>MSGLADASGPRDTQALLSATQAMDLRRRDYHMERPLLNQEHLEELGRWGSAPRTHQWRTWLQCSRARAYALLLQHLPVLVWLPRYPVRDWLLGDLLSGLSVAIMQLPQGLAYALLAGLPPVFGLYSSFYPVFIYFLFGTSRHISVGTFAVMSVMVGSVTESLAPQALNDSMINETARDAARVQVASTLSVLVGLFQVGLGLIHFGFVVTYLSEPLVRGYTTAAAVQVFVSQLKYVFGLHLSSHSGPLSLIYTVLEVCWKLPQSKVGTVVTAAVAGVVLVVVKLLNDKLQQQLPMPIPGELLTLIGATGISYGMGLKHRFEVDVVGNIPAGLVPPVAPNTQLFSKLVGSAFTIAVVGFAIAISLGKIFALRHGYRVDSNQELVALGLSNLIGGIFQCFPVSCSMSRSLVQESTGGNSQVAGAISSLFILLIIVKLGELFHDLPKAVLAAIIIVNLKGMLRQLSDMRSLWKANRADLLIWLVTFTATILLNLDLGLVVAVIFSLLLVVVRTQMPHYSVLGQVPDTDIYRDVAEYSEAKEVRGVKVFRSSATVYFANAEFYSDALKQRCGVDVDFLISQKKKLLKKQEQLKLKQLQKEEKLRKQAASPKGASVSINVNTSLEDMRSNNVEDCKMMVSSGDKMEDATANGQEDSKAPDGSTLKALGLPQPDFHSLILDLGALSFVDTVCLKSLKNIFHDFREIEVEVYMAACHSPVVSQLEAGHFFDASITKKHLFASVHDAVTFALQHPRPVPDSPVSVTRLALEVLFQ[2x]

Members of the SLC26 family constitute a conserved class of anion transport proteins, which encompasses uncoupled transporters with channel-like properties, coupled exchangers and motor proteins. Here we have determined the structure of the closely related human transporter SLC26A6 and characterized it as a coupled exchanger of chloride with bicarbonate and presumably also oxalate. SLC26A6 is widely expressed in different tissues including the heart, kidney, pancreas, and intestine. We also attempted to follow electrogenic Cl-/oxalate exchange by patch clamp electrophysiology in the whole cell configuration but did not measure pronounced currents that would be above background, likely due to the slow kinetics of the process. Together, our functional experiments characterize SLC26A6 as a strictly coupled transporter that exchanges Cl- with HCO3- and presumably also oxalate at a 1:1 stoichiometric ratio.

To reveal the molecular basis of the described transport properties of SLC26A6, we have determined its structure by cryo-electron microscopy (cryo-EM). A dataset of the protein purified in the detergent glycol-diosgenin (GDN) at 3.3 Å was of high quality and allowed for the unambiguous interpretation of the cryo-EM density by an atomic model (Figure 2—figure supplements 1 and 2). The structure defines an inward-facing conformation of the protein that generally resembles known structures of SLC26A9. In the homodimeric protein, subunit interactions are predominantly formed by the domain-swapped cytoplasmic parts including an extended N-terminal region and the C-terminal STAS domain, whereas the few contacts between the transmembrane transport units are confined to the end of the terminal membrane-spanning helix α14. The substrate binding site located in the center of the core domain is accessible from the cytoplasm via a spacious aqueous cavity, whereas the extracellular exit is sealed by extended contacts between core and gate domains. The presumable location of a bound chloride ion is resolved in the structure of SLC26A6 at a low contour of the map. The anion binding site is placed between the opposed short helices α3 and α10, which partly span the membrane and whose N-termini are aligned to face each other in the center of the core domain. In SLC26A9, Cl- binds in a deep pocket with low field strength, whereas the same pocket is shallower in SLC26A6, where a conserved arginine (Arg 404) increases the positive electrostatic potential and thus likely stabilizes the bound anion. In addition to its structural role, Arg 404 likely also contributes to the stabilization of bound anions by coulombic interactions, with its guanidium group potentially engaging in direct interactions with bicarbonate or oxalate. In the density, the N-terminal part of the IVS folds into an α-helix encompassing amino acids 569–593 (CαIVS) whereas the following 61 residues are unstructured and thus not resolved in the density.> MGIQGLAKLIADVAPSAIRENDIKSYFGRKVAIDASMSIYQFLIAVRQGGDVLQNEEGETTSHLMGMFYRTIRMMENGIKPVYVFDGKPPQLKSGELAKRSERRAEAEKQLQQAQAAGAEQEVEKFTKRLVKVTKQHNDECKHLLSLMGIPYLDAPSEAEASCAALVKAGKVYAAATEDMDCLTFGSPVLMFHLTASEAKKLPIQEFHLSRILQELGLNQEQFVDLCILLGSDYCESIRGIGPKRAVDLIQKHKSIEEIVRRLDPNKYPVPENWLHKEAHQLFLEPEVLD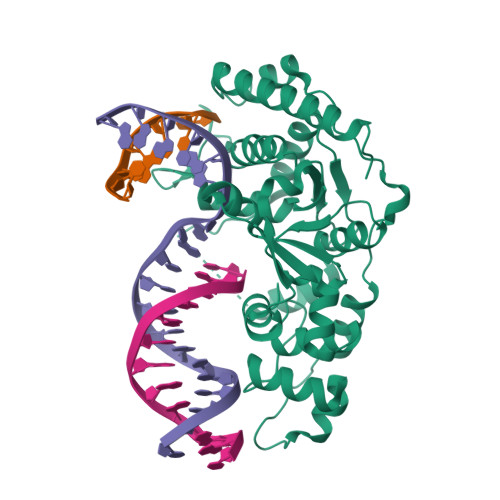PESVELKWSEPNEEELIKFMCGEKQFSEERIRSGVKRLSKSRQKLAAALEHHHH4-[(9-cyclopentyl-7,7-difluoro-5-methyl-6-oxo-6,7,8,9-tetrahydro-5H-pyrimido[4,5-b][1,4]diazepin-2-yl)amino]-3-methoxy-N-(1-methylpiperidin-4-yl)benzamide | C27 H35 F2 N7 O3 | 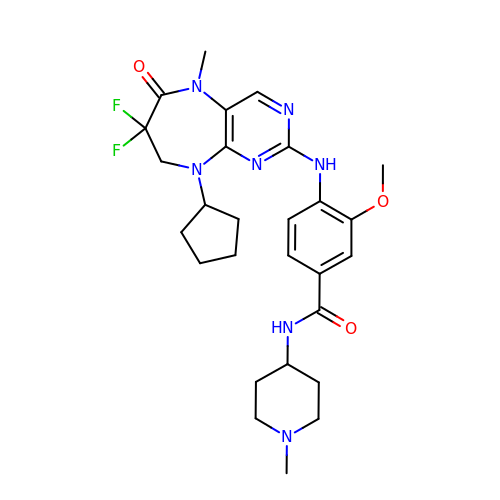DJNZZLZKAXGMMC-UHFFFAOYSA-N>MVGGVVIA[8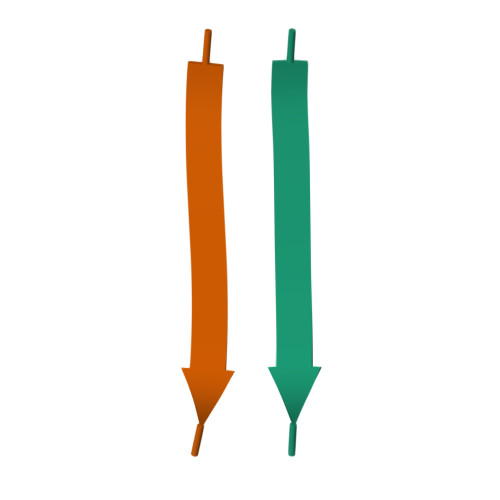x]GLUTARIC ACID | C5 H8 O4 | 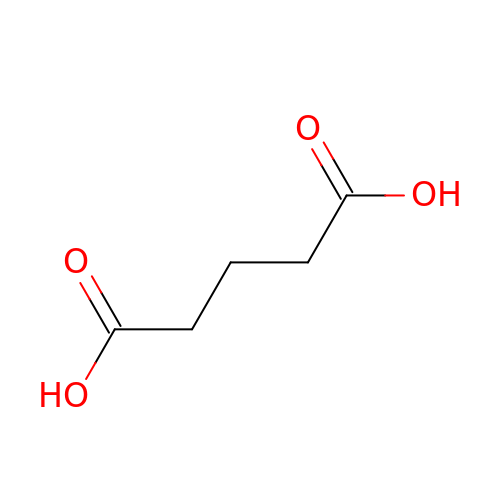JFCQEDHGNNZCLN-UHFFFAOYSA-N>[2x]MSLKAIGFEQPFKLSDGNLFKTFNLDIPEPKVHEILVKIQSISVNPVDTKQRLMDVSKAPRVLGFDAIGVVESVGNE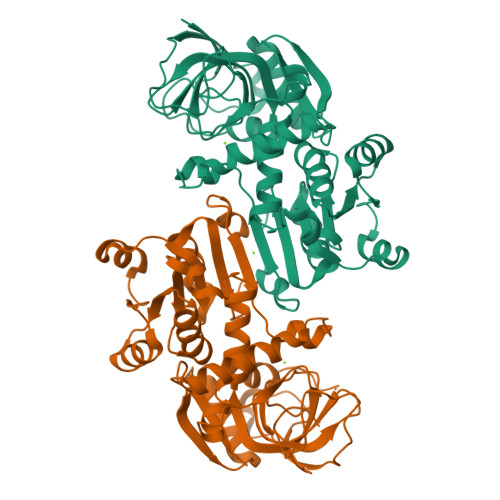VTMFNQGDIVYYSGSPDQNGSNAEYQLINERLVAKAPKNISAEQAVSLPLTGITAYETLFDVFGISRNRNENEGKTLLIINGAGGVGSIATQIAKAYGLRVITTASRNETIEWTKKMGADIVLNHKESLLNQFKTQGIELVDYVFCTFNTDMYYDDMIQLVKPRGHIATIVAFENDQDLNALKPKSLSFSHEFMFARPLNQTDDMIKHHEYLEDITNKVEQNIYQPTTTKVIEGLTTENIYQAHQILESNTMIGKLVINLNEGHHHHHH>GMGSMAEKWEELSGKNNWEGLLNPLDLDLRKYIIQYGELAQATYDTFISERASKYAGASRYSMENFFTKVGLDPSKYHVTKFFYGTSSIPLPDAFMTRSLSREAWSKESNFMGWIAVATDEGKVALGRRDIVINWRGTLQVLEWVNDLQFLLVPAPKVFGDGGLLPLFHPLVHHGFH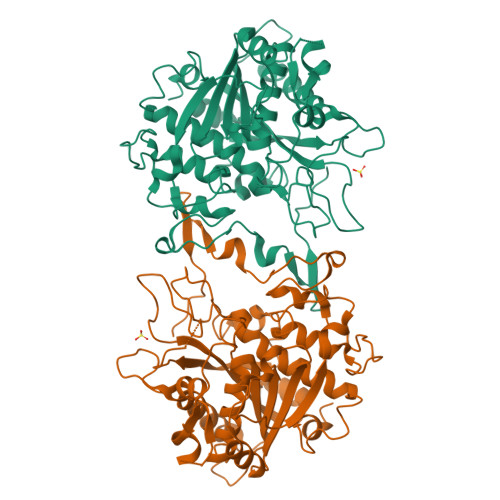NIYTTENPRSQFNKTCVRDQVMEEVKRLVEEYKNEEVSITVTGHSLGASLATLNAVDIAFNGINKSSNGKEFPVTAFVFASPKVGDLNFHKAFSKLKHLHILRIHNLLDIVPKYPPVGYFDVGQELMIDTTKSPYVKPPGEVVSWHLLEPYLHGIAGTQGIGMTAGFKLEVNRDISLVNKQWMILKDEYCIPPLWWSEKHKGMVQQQDGSWLLQDRDDYEF[4x]>MRVQSKGFAIFSKDEHFKPHDFSRHAVGPRDVLIDILYAGICHSDIHSAYSEWKEGIYPMIPGHEIAGIIKEVGKGVKKFKIGDVVGVGCFVNSCKACKPCKEHQEQFCTKVVFTYDCLDSFHDNEPHMGGYSNNIVVDENYVISVDKNAPLEKVAPLLCAGITTYSPLKFSKVTKGTKVGVAGFGGLGSMAVKYAVAMGAEVSV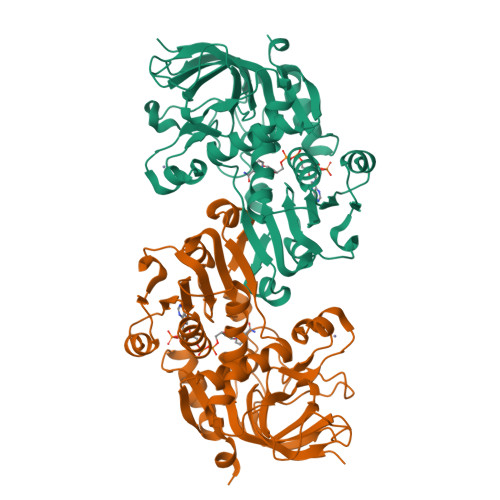FARNEHKKQDALSMGVKHFYTDPKQCKEELDFIISTIPTHYDLKDYLKLLTYNGDLALVGLPPVEVAPVLSVFDFIHLGNRKVYGSLIGGIKETQEMVDFSIKHNIYPEIDLILGKDIDTAYHNLTHGKAKFRYVIDMKKSFD[2x]>[4x]GSERQILRLKQINIQLATKIQHLEF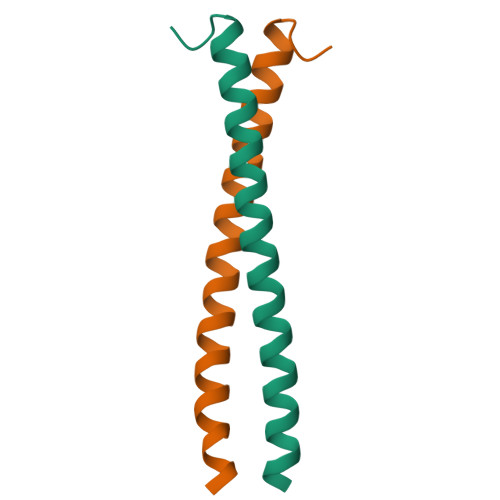SCSEKEQEIERLNKLLKQNGLLG> GPLGSVVRAKFNFQQTNEDELSFSKGDVIHVTRVEEGGWWEGTHNGRTGWFPSNYVREI;> GGFKPSRPPRPSRPPPPTPRRPAS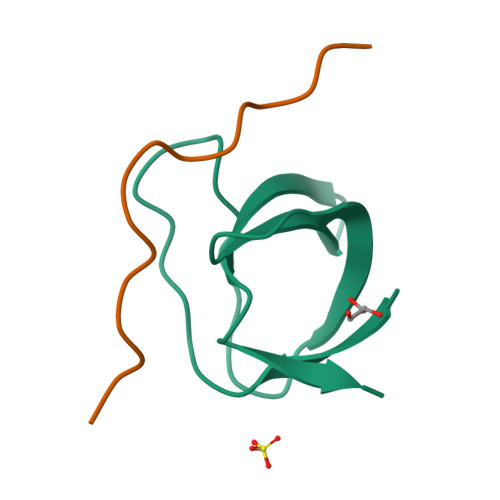V> TYPEGSPVYHNGKLSVQGTQMVSECGKPVQLRGMSSHGLAWFPKCYTEASLTALVKDWNIDIFRLAIYTHEWGGYTTNQWKSKDDYNAYIDNMVDICAKLGIYCIIDWHVLNDGSGDPNYTLDDAIPFWDYMSAKHKDDKHVLYEICNEPNGFDVKWADVKEYAEAVIPVIRKNDPDKIIICGTPTWSQDVDLAAQDPLSYDNVMYTLHFYSGTHTQYLRDKAQVAINKGLALFVTEFGTTQASGDGGVYFDECNTWMDWMDARKISWVNWSFADKPESSAALKPGASNSGDWNMVSESGQYIKRKLSQPKSYES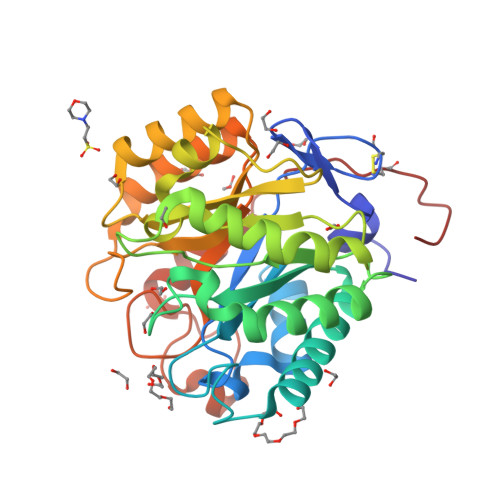CGGHHHHH>GIDPFTMNAAAEAEFNILLATDSYKVTHYKQYPPNTSKVYSYFECREKKTENSKVRKVKYEETVFYGLQYILNKYLKGKVVTKEKIQEAKEVYREHFQDDVFNERGWNYILEKYDGHLPIEVKAVPEGSVIPRGNVLFTVENTDPECYWLTNWIETILVQSWYPITVATNSREQKKILAKYLLETSGNLDGLEYKLHDFGYRGVSSQETAGIGASAHLVNFKGTDTVAGIALIKKYYGTKDPVPGYSVPAAEHSTITAWGKDHEKDAFEHIVTQFSSVPVSVVSDSYDIYNACEKIWGEDLR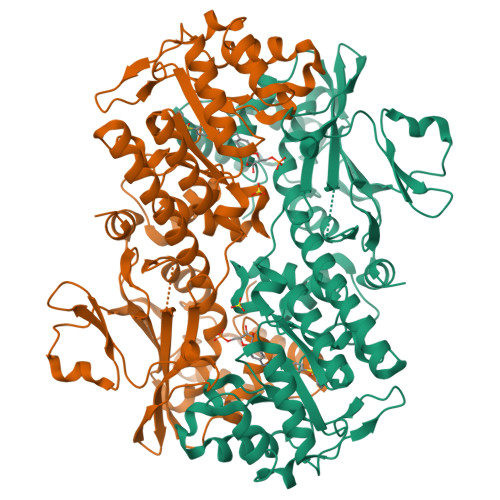HLIVSRSTEAPLIIRPDSGNPLDTVLKVLDILGKKFPVTENSKGYKLLPPYLRVIQGDGVDINTLQEIVEGMKQKKWSIENVSFGSGGALLQKLTRDLLNCSFKCSYVVTNGLGVNVFKDPVADPNKRSKKGRLSLHRTPAGNFVTLEEGKGDLEEYGHDLLHTVFKNGKVTKSYSFDEVRKNAQLNIEQDVAPH[2x]>[2x]MGSSHHHHHHSSGRENLYFQGMIYMPIVVAVDKKSDRAERVLRFAAEEARLRGVPVYVVHSLPGGGRTKDEDIIEAKETLSWAVSIIRKEGAEGEEHLLVRGKEPPDDIVDFADEVDAIAIVIGIRKRSPTGKLIFGSVARDVILKANKPVICIK

Universal stress proteins (USP) are widely spread proteins in nature. In stress conditions such as heat shock, nutrient starvation, the presence of oxidants, uncouplers, DNA-damaging agents, or other stress agents which may arrest cell growth, USP constitute a natural biological defense mechanism. Under stress, USPs are overproduced and through a variety of mechanisms aid the organism in surviving in such uncomfortable conditions. Here, we present the structures of both apo- and cofactor-bound forms of an euryarchaeal USP AF0826 from A. fulgidus and a bacterial USP NE1028 from N. europaea.

Based on this observation, we hypothesized that soaking or cocrystallization of that protein with ATP could result in formation of a crystal with the ligand bound in this region. As a result, we obtained the structure of AF0826 with dAMP bound in the vicinity of the ATP-binding motif. All of the residues binding dAMP in AF0826 are analogs of the residues binding AMP in the NE1028 structure, and interact with the ligand in very similar ways, as shown in Fig. 4B and D. Where hydroxyl groups are interacting with G and A (AF0826: G103, A9; NE1028: G114, A10) and adenine ring is positioned by either V or S (S40 and V40, respectively). AF0826 displays the same type 1 dimerization, the dimerization interface is formed by β5 and α4 from each monomer as it takes place is case of NE1028.> MEVKELERDKNRVVLEYVFGAEEIAQAEDKAVRYLNQRVEIPGFRKGRIPKNVLKMKLGEEFQEYTLDFLMDLIPDTLKDRKLILSPIVTERELKDVTARVVVEVHEEPEVRIGDISKIEVEKVDEEKVLEKYVERRIEDLRESHALLEPKEGPAEAGDLVRVNMEVYNEEGKKLTSREYEYVISEDEDRPFVKDLVGKKKGDVVEIEREYEGKKYTYKLEVEEVYKRTLPEIGDELAKSVNNEFETLEQLKESLKKEGKEIYDVEMKESMREQLLEKLPEIVEIEISDRTLEILVNEAINRLKREGRYEQIVSSYESEEKFREELKERILDDIKRDRVIEVLAQEKGISVNDEELEKEAEELAPFWGISPDRAKSLVKARQDLREELRWAILKRKVLDLLLQEVKVKVV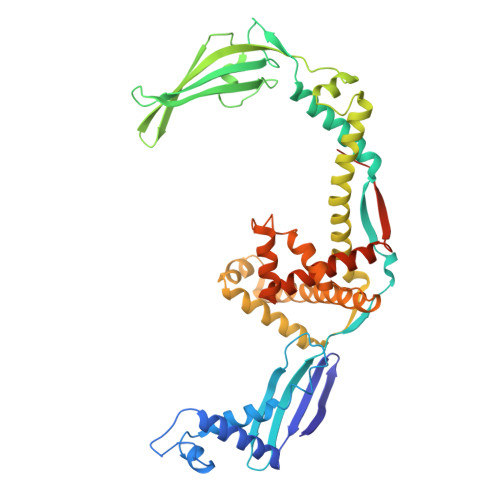EPKGEGDDSEGKEDNLEHHHHHH>GAMVSQPIKLLVGLANPGPEYAKTRHNAGAWVVEELARIHNVTLKNEPKFFGLTGRLLINSQELRVLIPTTFMNLSGKAIAALANFYQIKPEEIMVAHDELDLPPGVAKFKQGGGHGGHNGLKDTISKLGNNKEFYRLRLGIGHPGHADKVAGYVLGKAPAKEQECLDAAV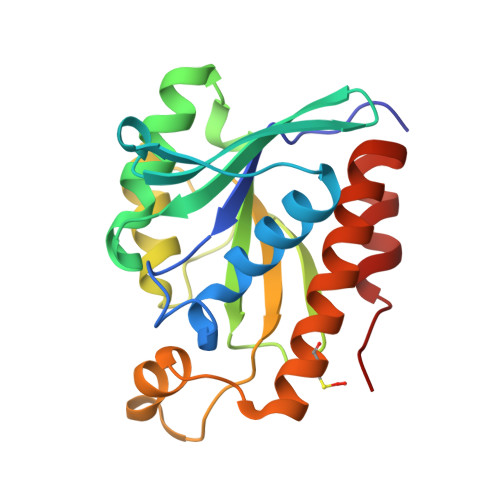DESVRCLEILMKDGLTKAQNRLHTFKAE[2x]>[8x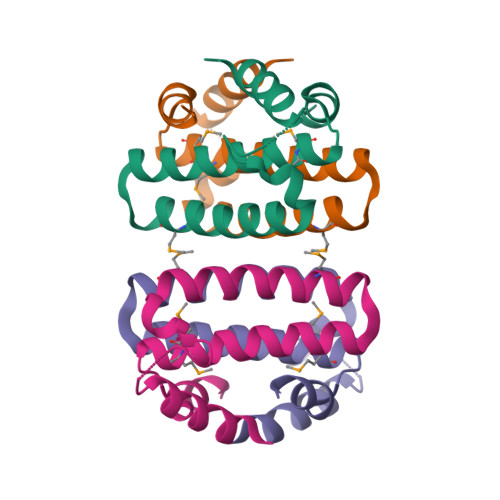]MSKKTFEELFTELQHKAANGDPATSRTAELVDKGVHAIGKKVVEEAAEVWMAAEYEGKDAAAEEISQLLYHVQVMMVARGISLDDVYAHLLEHHHHHH>[4x]MHHHHHHTSKIEQPRWASK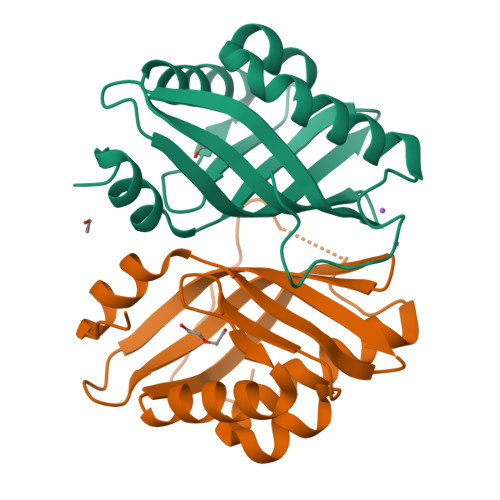DSAAGAASTPDEKIVLEFMDALTSNDAAKLIEYFAEDTMFQAMPLPPAYGRDAVEQTLAGLFTVMSIDAVETFHIGSSNGLVYTERVDVLRALPTGKSYNLSILGVFQLTEGKITGWRDYFDLREFEEAVDLPLRG>[2x]MHHHHHHGSTSLYKKAGSETLYIQGDHLPMPKFGPLAGLRVVFSGIEIAGPFAGQMFAEWGAEVIWIENVAWADTIRVQPNYPQLSRRNLHALSLNIFKDEGREAFLKLMETTDIFIEASKGPAFARRGITDEVLWQHNPKLVIAHLSGFGQYGTEEYTNLPAYNTIAQAFSGYLIQNGDVDQPMPAFPYTADYFSGLT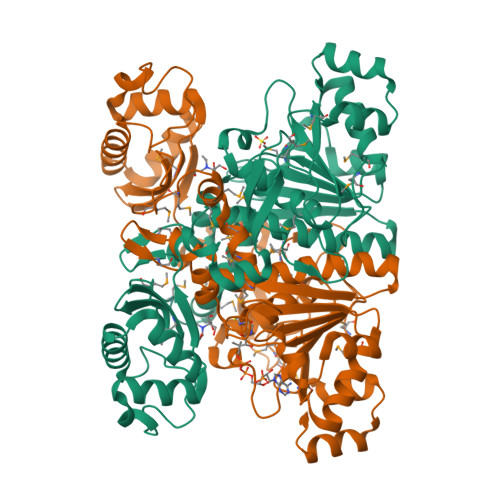ATTAALAALHKVRETGKGESIDIAMYEVMLRMGQYFMMDYFNGGEMCPRMSKGKDPYYAGCGLYKCADGYIVMELVGITQIEECFKDIGLAHLLGTPEIPEGTQLIHRIECPYGPLVEEKLDAWLATHTIAEVKERFAELNIACAKVLTVPELESNPQYVARESITQWQTMDGRTCKGPNIMPKFKNNPGQIWRGMPSHGMDTAAILKNIGYSENDIQELVSKGLAKVEDSTHHHHHH7-[(4-methylpiperazin-1-yl)methyl]-4-[(3-methyl-1H-pyrazol-5-yl)amino]-2-(tetrahydro-2H-pyran-4-yl)phthalazin-1(2H)-one 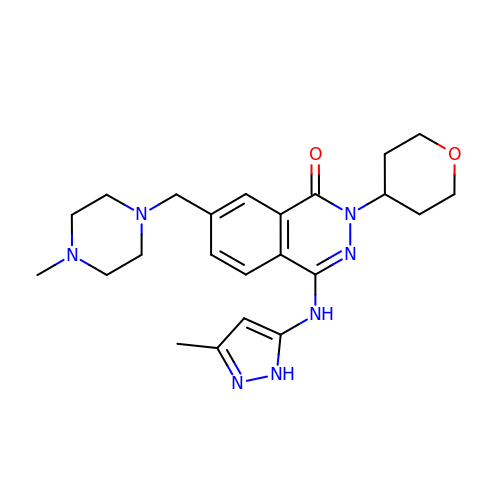| C23 H31 N7 O2 | IYIPJBAPGVUHNG-UHFFFAOYSA-N>MVRKGEKKLAKPPTTKAANPQPRRRANNRRRSNRTDAPVSKASTVTGFGRGTNDVHLSGMSRISQAVLPAGTGTDGYVVVDATIVPDLLPRLGHAARIFQRYAVETLEFEIQPMCPANTGGGYVAGFLPDPTDNDHTFDALQATRGAVVAKWWESRTVRPQYTRTLLWTSSGKEQRLTSPGRLILLCVGNNTDVVNVSVLCRWSVRLSVPSLETPEETTAPIMTQGSLYNDSLSTNDFKSILLGSTPLDIAPDGAVFQLDRPLSIDYSLGTGDVDRAVYWHLKKFAGNAGTPAGWFRWGIWDNFNKTFTDGVAYYSDEQPRQILLPVGTVCTRVDSEN[3x]

Nervous necrosis virus (NNV), a simple nonenveloped virus in the genus of betanodavirus, infects fish and damages aquaculture worldwide. The structure of GNNV VLP unveils GNNV capsid is a T = 3 icosahedral particle with a diameter of ∼35 nm and delineates the CP as consisting of three domains: an N-terminal arm, a shell domain (S-domain), and a protrusion domain (P-domain). The S-domain comprises an eight-stranded β-sheet to form a canonical “jelly-roll” structure as the building unit of virus capsid; three P-domains from contiguous CPs in one asymmetric unit are located outside of the capsid, presenting a protrusion at the quasi-3-fold axis. NNV uses protrusions to bind to common receptors of sialic acids on the host cell surface to initiate its entry via the endocytic pathway.

Specifically, we examined three pH points: weakly alkaline (pH 8.0) for host cell docking, weakly acidic (pH 6.5) in the early endosome, and acidic (pH 5.0) in the late endosome. By using three-dimensional (3D) reconstruction with icosahedral symmetry, we determined cryo-EM structures of GNNV VLPs at pH 8.0, 6.5, and 5.0, as well as virions at pH 6.5 and 5.0, with overall resolutions in the range of 2.82–4.36 Å. Cryo-EM images revealed a spikier appearance of the GNNV VLPs at pH 8.0 and 6.5 than at pH 5.0. Our cryo-EM results show the protrusions on GNNV adopt erect/loose configuration at pH 8.0 and 6.5 but become prone/compact at pH 5.0. Notably, the diameter of the GNNV particle under acidic conditions (pH 5.0) was smaller (370 Å) than under weakly alkaline (pH 8.0) or neutral (pH 6.5) conditions (380 Å). Thus, our cryo-EM imaging has revealed that GNNV structures are pH-responsive for the first time, with protrusions on GNNV adopting an erect position under weakly alkaline and neutral conditions but a prone position under acidic conditions. GNNVs dock on their host cells, e.g., Grouper fin cells, under weakly alkaline conditions as wild Groupers live in relatively warm oceanic regions that exhibit weakly alkaline conditions (pH 8.1) or under neutral conditions (pH 7.0–7.5) for farmed Grouper. By mimicking those conditions encountered en route of host cell entry via the endocytic pathway, we discovered that the protrusions on the GNNV capsid adopts an erect/rising position with loose configuration at the docking condition (pH 8.0) and early endosome condition (pH 6.5), but compact and rest on the capsid shell at the late endosome condition (pH 5.0).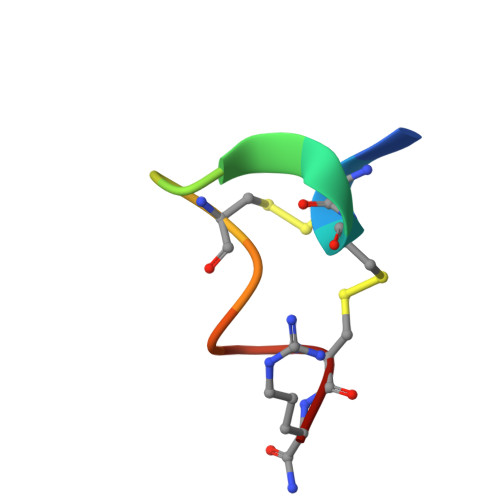> GCCSDPRCRYRCR>[2x]METDTLLLWVLLLWVPGSTGDAAQPARRANGSEWSYTNILTGPETWHEHYKNMCSGYYQSPIDLKTDISTLDLKLKTVIIY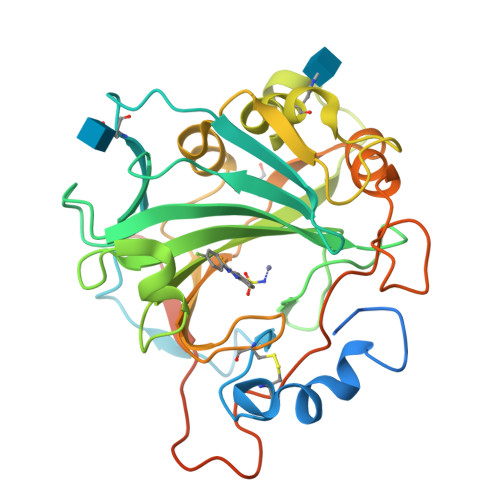RNTSSTETTTIQNNGHSAEVKFPRNTWFISFDGILDYKYEIIQMHFHWGNTDDRGSEHTIDGFRFPLEGHIVSFRRQMYSSPSEAIGRPGGLAVLGIMHQIVESIKYEQTAFKAYNNFSGVLNSQFVPPNNSTIDDINLALLLSLLNPSRYFRYLGSLTTPPCTENVLWTVFIDPVLITREQINLFRNLPYGSNEKQTRMGDNFRPIQLLNPIDTLASRTLYRATARGGPEQKLISEEDLNSAVDHHHHHH>MRCIGISNRDFVEGVSGGSWVDIVLEHGSCVTTMAKNKPTLDFELIKTEAKQPATLRKYCIEAKLTNTTTDSRCPTQGEPTLNEEQDKRFVCKHSMVDRGWGNGCGLFGKGGIVTCAMFT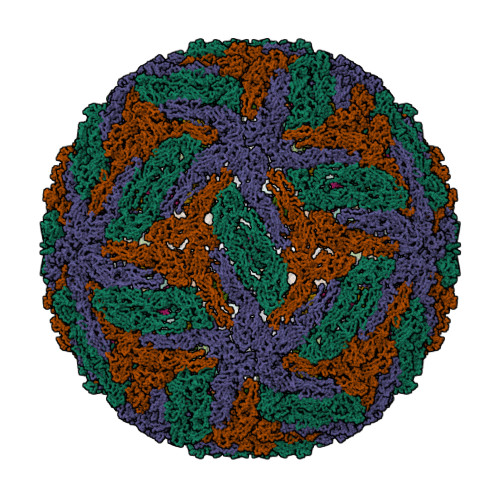CKKNMEGKIVQPENLEYTVVITPHSGEEHAVGNDTGKHGKEVKITPQSSITEAELTGYGTVTMECSPRTGLDFNEMVLLQMKDKAWLVHRQWFLDLPLPWLPGADTQGSNWIQKETLVTFKNPHAKKQDVVVLGSQEGAMHTALTGATEIQMSSGNLLFTGHLKCRLRMDKLQLKGMSYSMCTGKFKVVKEIAETQHGTIVIRVQYEGDGSPCKIPFEIMDLEKRHVLGRLITVNPIVTEKDSPVNIEAEPPFGDSYIIIGVEPGQLKLDWFKKGSSIGQMFETTMRGAKRMAILGDTAWDFGSLGGVFTSIGKALHQVFGAIYGAAFSGVSWTMKILIGVIITWIGMNSRSTSLSVSLVLVGIVTLYLGVMVQA[3x];>[3x]SVALVPHVGMGLETRTETWMSSEGAWKHAQRIETWILRHPGFTIMAAILAYTIGTTHFQRVLIFILLTAIAPSMT>[10x]MEGLNLVATALAVGLGAIGPGVGIGIIVSGAVQAIGRNPEIENRVVTYMFIGIAFTEALAIFGLVIAFLIGFGVLQ;>[2x]MSTRTRNILIIVGALIISIASRFFLYTGPPHVEVAAEVIFDGIPGFPITNSFVVAIIIDIFVIALAVAATRNLQMVPRGLQNVMEFILESLYNLFRNINAKYVATAFPLVATIFLFVLFGNWFGLLPGVGSIGVCHEKKEEHAVVDERLALAAPAAPLSSVAAAEGEEIHDTCAAQGKKLVPLFRAPAADLNFTFAIAVISFVFIEYWGFRALGPGYLKKFFNTNGIMSFVGIIEFISELVKPFALAFRLFGNIFAGEVLLVVMAFLVPLLLPLPFYGFEVFVGFIQALIFALLTYAFLNIAVTGHDEEHAH;>[4x]MEALGINPTLFIAQLINFLLLIFILRALLYRPVMNLLNERTRRI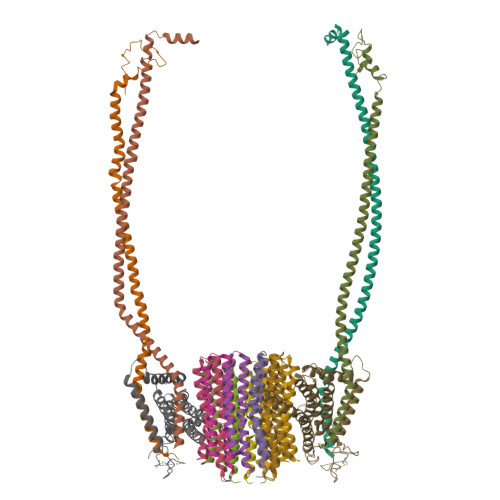EESVRDAEKVREQLANARRDYEAEIARARQEAAKIVAQAQERAKQQEAEIIAQARREAERLKEEARAQAEQERIRMLSEAKSQIADLVTLTASRVLGAELQARGHDALIAESLAALDRRN>VSSRVSTRSSLAEDLRAIGLADGDAVLVAAALRKVGKIVGGPDDILDAMRDVIGPAGTVLGYADWQLEDEIRDDPAMREHIPAFDPLRSRSIRDNGFWPELIRTTPGALRSASPGASMAAIGGEAEWFTADHALDYGYGPRSPLGKLVEAKGKVLMLGAPLDTMTLLHHAEHLADFPNKRILRYEAPILVDGEKVWRWFEEFDTSDPPDGLADDYFAGIVEEFLATGRGKRGKIGEASSVLVPADEIVAFAVDWLERWGRTAR[6x]

Here, we conduct a comprehensive functional analysis of the Antibiotic_NAT family of aminoglycoside acetyltransferases. AG resistance is primarily conferred by three classes of aminoglycoside-modifying enzymes (AMEs): phosphotransferases (APHs), nucleotidylyltransferases (ANTs), and acetyltransferases (AACs). AMEs permanently alter the AG substrate, preventing them from binding to their target, the A-site of the 16S rRNA in the bacterial ribosome. The fold typical of the Antibiotic_NAT family is evident in all structures, composed of 13 α-helices and 8 β-strands, and determined structures superpose with pairwise RMSD’s 0.8–1.0 Å between 197 to 266 matching Cα atoms.

The meta-AAC0038 adopts a dimeric structure with a buried surface of ~900 Å2 per subunit. This enzyme also forms a dimer in solution according to the size exclusion chromatography (not shown). Similar sequence signatures (residues Thr165-Glu171 in meta-AAC0038) were identified in all analyzed members of this family, with His and Glu (His168 and Glu171 in meta-AAC0038) along with two glycine residues (Gly122 and Gly158 in metaAAC0038), completely conserved. This motif’s threonine (Thr165 in meta-AAC0038) is also conserved in all but one of the analyzed sequences where it is substituted by a chemically similar serine.(S)-N-(5-chloro-3-((4-(cyclopentanecarbonyl)-3-methylpiperazin-1-yl)methyl)-2-methylphenyl)-2-methylpyrimidine-5-carboxamide 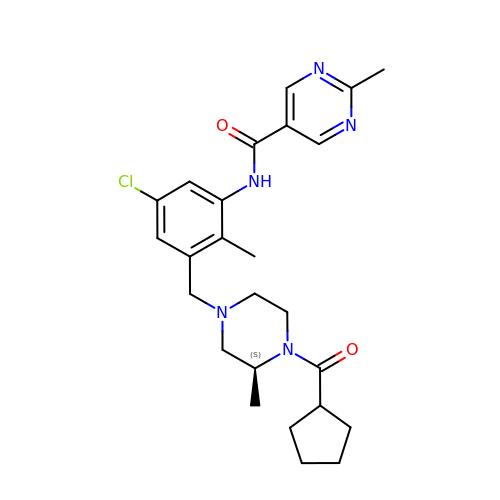| C25 H32 Cl N5 O2 | HAXBJJXPLDXDIL-INIZCTEOSA-N>MSLQTKILIIDGDKDNCQKLKGFLEEKGISIDLAYN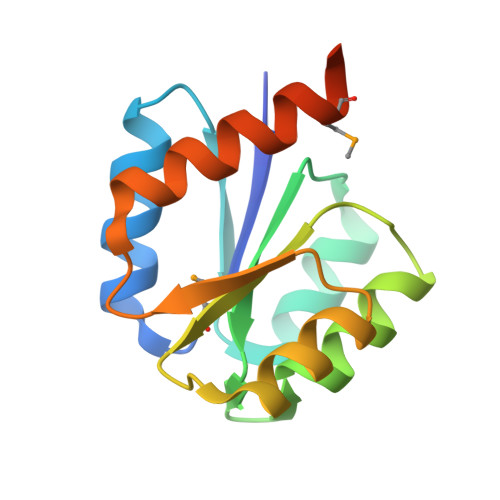CEEAIGKIFSNKYDLIFLEIILSDGDGWTLCKKIRNVTTCPIVYMTYINEDQSILNALNSGGDDYLIKPLNLEILYAKVKAILRRMNSYVNNEGHHHHHH[6x]> CGGUGUAAGUGCAGCCCGUCUUACACCGUGCGGCACAGCGGAAACGCUGA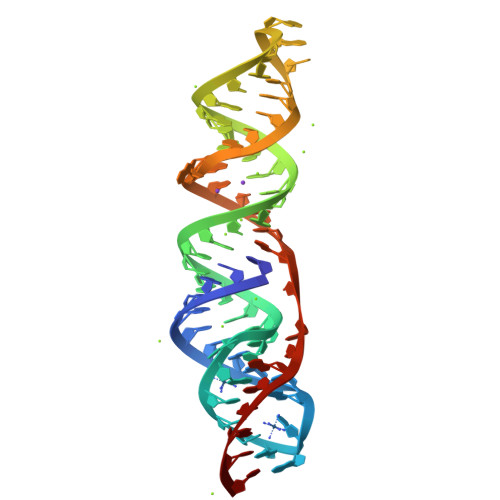UGUCGUAUACAGGGCU Parkin is an E3 ubiquitin (Ub) ligase of the structurally uncharacterized RING-in-between-RING(IBR)-RING (RBR) family, which, in an HECT-like fashion, forms a catalytic thioester intermediate with Ub. In RBR E3 ligases, a RING domain (RING1) mediates transfer of Ub from the E2 to a catalytic Cys of the RING2 domain, from which Ub is subsequently transferred to a substrate. PINK1 senses damaged mitochondria, and recruits and activates Parkin to ubiquitinate mitochondrial outer membrane proteins including mitofusins and Miro. A C-terminal RBR domain comprises an E2-binding RING1 domain, an IBR domain and a RING2 domain that contains the catalytic Cys residue (Cys431) for E2-mediated Ub charging.

We generated sufficient yields of soluble protein from human Parkin construct spanning aa 137–465, which was codon-optimized for expression in E. coli. Purified protein was crystallized and the structure was determined to 2.25 Å resolution using the anomalous signal of the eight coordinated zinc atoms from a single anomalous dispersion experiment. The structure of human Parkin UPD-RBR revealed four domains with unanticipated inter-domain interactions. Central to the structure is the UPD (aa 142–227), a previously undescribed elongated Zn-binding fold in which two central anti-parallel β-strands arrange two Zn-coordinating loops. The RING1 domain of Parkin (aa 228–327) is a variation of the canonical RING fold. The C-terminal RING2 domain shows a fold that does not resemble RING domains but rather the Parkin IBR domain. Parkin terminates with a C-terminal Trp462-Phe-Asp-Val465 motif, which is the centrepiece of an extensive (686 Å2) hydrophobic interface with the UPD. Importantly, Cys431 is also located at the interface, buried from solvent, and inaccessible for transthiolation. Superposition of Parkin with RING-E2 complex structures revealed significant steric clashes of E2 with the Parkin linker helix that connects IBR and RING2, as this binds RING1 across its E2 and Ub binding sites. Hence, our structure suggests that the linker helix between IBR and RING2 inhibits E2 and E2∼Ub interaction with RING1.

> PAGRSIYNSFYVYCKGPCQRVQPGKLRVQCSTCRQATLTLTQGPSCWDDVLIPNRMSGECQSPHCPGTSAEFFFKCGAHPTSDKETSVALHLIATNSRNITCITCTDVRSPVLVFQCNSRHVICLDCFHLYCVTRLNDRQFVHDPQLGYSLPCVAGCPNSLIKELHHFRILGEEQYNRYQQYGAEECVLQMGGVLCPRPGCGAGLLPEPDQRKVTCEGGNGLGCGFAFCRECKEAYHEGECSAVFEASGTTTQAYRVDERAAEQARWEAASKETIKKTTKPCPRCHVPVEKNGGCMHMKCPQPQCRLEWCWNCGCEWNRVCMGDHWFDV>[2x]VNGTFVESIADAHVELRAAMLGSRHHPSPDIPIINHPSASGLDQAFALVEASLTAHGLAIVQMDEPLSTEQFACYARRLGVLVPEHDEDV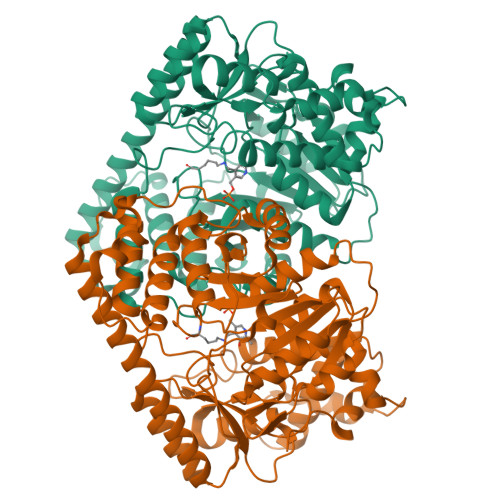QPFVEQGDILHLRTRFGPTDRVGLQPFSSSPLSMHSESSGNALVDQPRYLAFQCLEPGEFAYAPQTLLIDMASIVARISPYNINILARTYYDSQRNSPPLLRYDGQRWVISFRDFQQQPLSWVHEGPTPAGDVLSAIRDLLACMYTAQASAVRWARGMFMVFDNQRYMHARSKGHFVLDQQDRHLLRARIRARTPDLNVLAAVDDGDSRVLFARPASGRIPQLPDDFRQTSAVEPNQVEETPDTFIDERTLEVFSRALNPTNPMELRNLWLGRVEAELGDNALRPEYADLWRRSRVRRAVSVEEVLRSTATVGMVKELFNAFFRDDLYGALSSKRNIILSSGAVDEDEYGLPAALKETLRFALARNFYGYSDSLGRQPAREAVAAMESVSMQQGHYEAASVALTMGATHTISSLADFIFRDNPYADAAICAIPNYPPLVQSIAWRHPVLLVPTPSHGGTTSLQALSRAVTPNTPMVLLQTGTNPCGSLVDELELERFIQSTSLSTLIILDECHEWLGAPRHFSPARQRANVIRVSSLSKNWSVPGLKVGWFLADPALVSRYYEFASTSYGGPQSFVYTLVEVLARFERWIIEGRTSIDQQQLREFSASYGLQLGSLSQTYEHYVAERRAREQVLLGLRGEATSCLRRASMIVKTPQCSINVFAQIPGSEDSYLSFRNVLRETGVSVYPGILSFYLAGGGFRVTTARKWGDLHRGLERLSAGAGNA>STYNGPLSSHWFPEELAQWEPDSDPDAPFNRSHVPLEPGRVANRVNANADKDAHLVSLSALNRHTSGVPSQGAPVFYENTFSYWHYTDLMVYWAGSAGEGIIVPPSADVIDASHRNGVPILGNVFFPPTVYGGQLEWLEQMLEQEEDGSFPLADKLLEVADYYGFDGWFINQETEGADEGTAEAMQAFLVYLQEQKPEGMHIMWYDSMIDTGAIAWQNHLTDRNKMYLQNGSTRVADSMFLNFWWRDQRQSNELAQALGRSPYDLYAGVDVEARGTSTPVQWEGLFPEGEKAHTSLGLYRPDWAFQSSETMEAFYEKELQFWVGSTGNPAETDGQSNWPGMAHWFPAKSTATSVPFVTHFNTGSGAQFSAEGKTVSEQEWNNRSLQDVLPTWRWIQHGGDLEATFSWEEAFEGGSSLQWHGSLAEGEHAQIELYQTELPISEGTSLTWTFKSEHDNDLNVGFRLDGEEDFRYVEGEQRESINGWTQWTLPLDAFAGQTITGLAFAAEGNETGLAEFYTGQLAVGADSEKPAAPNVNVRQYDPDPSGIQLVWEKQSNVHHYRVYKETKHGKELIGTSAGDRIYIEGLVEESKQND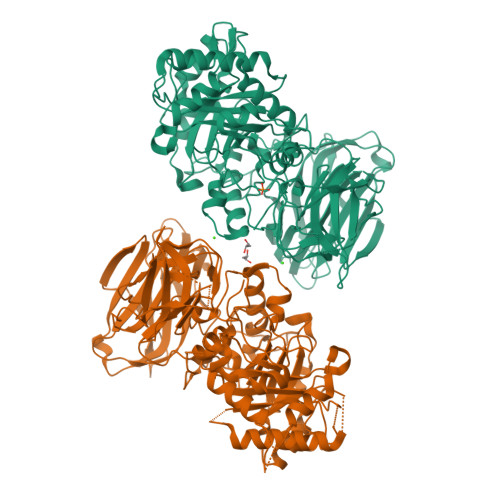VRLHIEALSETFVPSDARMIDIKSGSF[4x]> AAKALIVYGSTTGCTEYTAETIARELADAGYEVDSRDAASVEAGGLFEGFDLVLLGCSTWGDDSIELQDDFIPLFDSLEETGAQGRKVACFGCGDSSWEYFCGAVDAIEEKLKNLGAEIVQDGLRIDGDPRAARDDIVGWAHDVRGAI

Previous studies showed that proper introduction of disulfide bonds could stabilize the flexible region of target proteins and reduce the conformational entropy by locking the protein into single desired conformation. Here we developed a comprehensive disulfide bond prediction algorithm that not just increased the success rate of predictions but also improved the quality of crystallized target proteins. We applied our method on two proteins which were previously determined to high resolution and frequently used as fusion partners for GPCR crystallization, cytochrome b562 (BRIL) and Flavodoxin, and verified our prediction by solving the crystal structures of the wild type (WT) proteins and mutants. The theoretical and experimental results both indicated that with relatively lower values of conformational entropy, proteins would be more stable and readily crystallized to higher diffraction resolution.

The continued disulfide omitted electron densities of the side chains suggested that the disulfide bonds are successfully formed in all crystallized mutants, which are T9C-A36C, A20C-Q25C, V16C-A29C, and K27C-A79C in BRIL and N14C-C93, A43C-L74C, and C102-R125C in Flavodoxin, respectively. The WT and disulfide engineered Flavodoxin structures were determined to high-resolution of 1.20–1.55 Å with B-factors in the range of 16.15–19.24 Å2. On the other hand, the V16C-A29C and A20C-Q25C in BRIL, the N14C-C93 and A43C-L74C in Flavodoxin have higher entropy than that of WT counterparts, consistent with their relatively lower diffraction resolutions.> GHMESKKRQWALEDFEIGRPLGKGKFGNVYLAREKQSKFILALKVLFKAQLEKAGVEHQLRREVEIQSHLRHPNILRLYGYFHDATRVYLILEYAPLGTVYRELQKLSKFDEQRTATYITELANALSYCHSKRVIHRDIKPENL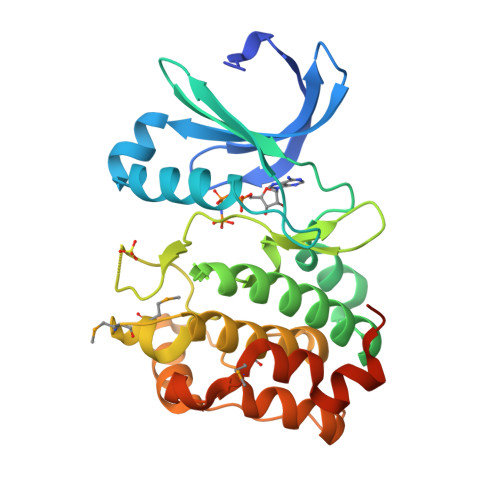LLGSAGELKIADFGWSVHAPSSRRTTLCGTLDYLPPEMIEGRMHDEKVDLWSLGVLCYEFLVGKPPFEANTYQETYKRISRVEFTFPDFVTEGARDLISRLLKHNPSQRPMLREVLEHPWITANSSKPSNCQNKESASKQS> MADRANNDDDVDRQPLPIADDADDDVDGIDEMFNNEDEDPEDEEGENLFGDDMERDYREQPELDQYSESGMDDASDVGSLSVSARRAAEREMAQRDQLLDDDALMYEDGDSEEVDTRRRGRGRRGRGDAADDDSVPMEEEDIPVDILENIRGRTIRDHVSDEAVAKEIERRFKNFLRSFHEPGNKQTKYIQMIKSMAADNRESLEVSFTDLSDDNGEQNISYFLPEAPNEMLAIMDRAATEVVMNMYPFYSRVCNEIKVRISQLPVEEDIRMLRQVHLNMLIRTAGVVTIASGILPQLAVVKYDCVACGYLLGPFVQQNDEEVRPTICPSCQGKGPFELNVENTVYHNYQRITMQESPNKVAAGRLPRSKDVILLGDLCDSCKPGDEIEVTGVYTNNFDGSLNYKQGFPVFNTLIHANHITNKDKMASDQLTDEDIKAIRELSQDPNISQRVFSSIAPSIYGHDDVKRAIALALFRGEAKNPGAKHRLRGDINVLLCGDPGTAKSQFLRYAAHIAPRSVLTTGQGASAVGLTAYVQRHPVTREWTLEAGAMVLADKGVCLIDEFDKMSDQDRTSIHEAMEQQSISISKAGIVTSLHARCTVIAASNPIGGRYNPTRTFAENVDLTEPILSRFDVLCVIRDSVDSVEDERLAKFVVGNHRTHHPDAKKIVKEGDELEEDQMDERTGVRLIPQDLLRKYIIYAREKCHPTLPEQHSEKFSNIFAQMRKESMATGSVAITVRHVESMIRLSEAHAKLHLRSYVNDEDCAAAIRVMLESFVNTQKASIMRMMKKTFSRHLTENRSANELLLFILKQLIRQQMHYATARAAAGTILQSVTIPESEFIEKAQQLRIENVKPFYTSEIFASNNFLYDPSKKTIVQEIF;> MDGQADGMFIDRAEDARKQEITEQYLNFLDNQADTFHYRQKIVKMMNDGESRLVMNLDEIREILPERAEGLLTQSVLEMNCLQSALQMAINRSDVQAVVKTGFHVGFEGTFGERHVNPRTLKSSYLGNLVCCEGIVTKCSTVRQKLLTSVHYCPATNKVLEKKFADFTMLDTAVTNNNYPTEDENKNPLETEFGHSVYKDHQTFTIQELPESAPAGQLPRAVDCVADLDLADRVKPGDRVRIIGVFRVLPNKQNGVSSGSFRSIIIINHIQMLSKEVIPNFEPQDVKDVRKISKSRNPFELLARSLAPSICGHEETKKALLCLLLGGMEKILNNGSRLRGDINVLLIGDPSVAKSQLLRYVLRMAPRAITTTGRGSSGVGLTAAVTTDPDSGERRLEAGAMVLADRGVVCIDEFDKMSDIDRTAIHEVMEQGRVTISKAGIHAKLNARCSVLAAANPVYGRYNPFKSPMENIGMQDSLLSRFDLIFVLLDEHDADKDANVAEHVLKLHTYRTQGEADGTVLPMGGGVETISTINMETKKASSSIYEENTQWAGIQDTKILTMDFMRKYIHLARSVQPKLTDEATEYISEVYADIRSFDITKTDQERTMPVTARQLETLIRLSTAIAKARFSKKVEREDTEKAYNLLHFACFKEKPKARQEYEKKKRAPRIDGDDDEDQSDNEDMATSEEPQSSSVPTAATPRRGVRRRAEDDDSQDSMMDTTIGESQPTAKKARTGPAAIGVDRYKELRKYVRKAFDDIGSTDDMVELQIITDSVQTQAGSHKFTEDELKAGYEQLENDNAAMIAEDKITLI;> MPRSNDPAEPQSESADLFAEPSSQHSSMRSGSEQVAGNMSPRSTSSASALQYGSEMGSVSQMSSASTLRRGGPRGDLGIAAVDHRTVQIRGMEDEMAGDDGQPRLYVWGTRICVADVQRSFRDFLTTFKISQLAEDENMMTGHDEALHEIDVNHPYYMERLLECNDAEVTHINLNLKHLNAFSEALYRKVIAYPADVIPYLDIVVNEVFAERFNRTLAQSIELRPFNAQKTRNMRGLNPNDVDQLITISGMVTRTSSLIPEMRSGYFQCAVCAFGIESEVDKGRIEEPVVCTNCSNTHCFQLVHNRSVFLDKQVVKLQESPDDMPSGETPHTVSVYAHGSLVESVQPGDRITVTGIFRATGMKVNPKQRALASVYRTSIDALHFRKMDTSRLHQDNGETITEERIQQIIELSKRPDIMDALAQSIAPSIYEHDDVKRGLLCLLFGGTRKDDETTNKTKLRSEINILLCGDPGTSKSQMLQYVYRLLPRSQYTSGKGSSAVGLTASVSRDADTKQLVLQTGALVLADNGVCCIDEFDKMNESARSVLHEVMEQQTLSIAKAGIICQLNARASVLAAANPVDSKWNRNKTIVENITLPHTLLSRFDLIFLIVDAQDEMQDRRLGNHLVSLYFENDGNQEKTEHVDMNLLRDYIAYAKANIHPKLSEEASQFIIEKYLFMRKAGAQHGQITAYPRQLESLIRLSEAHAKIRLSQEVSVDDVEKAFTLWREALKQSAVDPSTGRVDVAILASGMSASGRKAVEAMCEAVLKQLKTAKGFVTSKALFHTLKSADKTCQREVFDEAINELSKKESIARSGDRIRFQTEA;> MSNLDNPGIYYQERFFANDGVPDTGRELIAEYRQLITQFRNFIRDFSTGGFGMIYRDQLKRNYFSHEYRLEINLNHLKNFDEDIEMKLRKFPGKVLPALEEAAKIVADEITTPRPKGEEKLHDIQVTLTLDEYPTSLRQVKSAQVSQVVKISGIIVAAAQVRSKATKVTLQCRQCKHTIPDVSIKPGLEGFALPRTCAAPQQGQMQRCPIDPYIMLPDKCECVDYQTLKLQENPEDVPHGEMPRHLQLFTERYLTDKVVPGNRVTIVGVYSIKKLIQKKGGDKSLQGIRTPYLRVLGIHMETSGPGRTNFTTFTPEEERMFKTLAQRKDAYELIAKSIAPSIYGSADIKKSIACLLFGGARKKLPDGITRRGDINVLLLGDPGTAKSQLLKFVEQVSPIGVYTSGKGSSAAGLTASVIRDPQSRSFIMEGGAMVLADGGVVCIDEFDKMREDDRVAIHEAMEQQTISIAKAGITTTLNSRCSVLAAANSVYGRWDESRGDDNIDFMPTILSRFDMIYIVKDTHDVLKDATLAKHVIEVHVNASAAKERDIAGVPKTATTDSDGVMTMFDTDGFLTIEFLKKFVTYARLNCGPRLTPQASEKLVNHYVKMRNPVVNADAFKSGKKAHNSAIPITVRQLEAIVRIAESIAKMELQQFATDKHVEEALRLFRVSTIEAAATGNLAGVEGFTSTADQEALNRIEVQMKKRFAIGTHVSEHLIVQDFVARQHYRESLVKKVIDNLVRRGDLQQKMQRKMLYRVR;> MDNIIGGQAQQVEDTDGTRVQNEFSKFLKSFKDQKNEFIYKSAMKELVQPEKNTIFINMQHLYKFSNNLATTIELQYYRVYPFMCEALHLATLDACDESERQQMFKKQLYVSLFNLDAKTKVRELSADKVGGLVRIAGQIVRTHPVHPELSRACFVCEDCGVTTRDVQQQFRYTQPTKCANPQCMNRTRFSLDVNSSTFVDFQKIRIQETQAELPRGSIPRTVDVIVRGEMVETVQPGDKCDIVGTLIVIPDIAQLSTPGLRAETSNQNRGRATDKSEGITGLKALGVRDLTYKMAFLACHIQQTESLVGGDASGAVEETDYLDLWSKMSTEDRATLKKMSDDKKIEKNIVDSLFPNIYGNHEVKLGVLLMLLGGVAKKSRDEGTSLRGDINVCLVGDPSTAKSQVLKAVEEFSPRAIYTSGKASSAAGLTAAVVKDEESFEFVIEAGALMLADNGVCCIDEFDKMDLKDQVAIHEAMEQQTISITKAGVKATLNARASILAAANPVNGRYDRSRPLKYNVQMSAPIMSRFDLFFVLVDECNEVTDYAIARRILDNHRAISEHTERDSVYKIDDIKKYIAFARCFKPKISDKAAETLVREYKKLRMSDSNNAATSSWRITVRQLESLVRLSEALARLHCGKEVLVEHVEKAAELLNKSIVRVEQPDIALDDDDFDNNIMVVEADKENQRGDDSMDHDGEKENAPKIDIAKLKISFKEYKQLSDVLVLHMRSDEDNQGEDEYDGVKQSALVEWYLSTIEADLETEEDFNVQKTICERVIHRLIHQDHVLLEVEQGEDPTLCVHPNYVIADE;> MKTTTYNTDWAAEKTKIRSFFDEYYVDNEDGSGKAFPYRDQVFEIARRDKQAIVVNVDHIKESDIPDALELSEAITSNTKRYEVLFKDTISDMIQDYLGDKQAPVIDALDAYMFQRLHMDRNEGAANEEVSLQDKRKKYPPQLLQRFEVYFTTDDAAHETCVRNIKATEIGHLVSMKGVVIRATEVKPCVEVMTYTCDTCAAEVYQPVKGMQFTPPVNCPNKECVEAKANGRLHMQLRGSKFVKFQELKIQELSEQVPVGSIPRTMTVHVYGEMTRKCNTGNVVHVSGVFLPIMQSGFRPTGGLVADTYLEAHYINNLDDNPTFNGVQSAELEVLRRKGDNYETLAASIAPEIFGHVDVKKCLLMALVGGNDNSSNGMKIRGCINVLMMGDPGVAKSQLLGYVNRLAPRSQYTTGRGSSGVGLTAAVMKDPVTGEMSLEGGALVLADGGICCIDEFDKMMDHDRTAIHEVMEQQTISIAKAGIMTTLNARTAIIAAANPAYGRYNPNRSIEQNVDLPAALLSRFDLILLMQDKADRENDKILAEHITYVHQHGCHPNREKKDLISLETLREYISLCKTYTPTVDPALRERIVEAYVEMRRDARYSSDPTFVSPRMILGIVRMATARAKLRLSTIVDESDVEEALRLMQFAKDSLRPEQNKIEKRMAPVDAAFAVLRELYHADNAPIAISNAIQRCARKGISEVALKKCLDQYTANGLLVMDRQNIVFAMN;> GPGSMSSGDQNRGGVADKALQLVLEMKRNPDVLPPYNTELVRQCYQKIDELFQKNAAVVEKIRAGLPHDSTLLQPRLAAMCHIRRCMMAYVNERKNRIRSFRWKYGGALPASVRNALCDAEIQFFNEYSSTLARFQSNLGEGGVNLLLHSAPPKSLFVQVRALEDYGEFETSDGTQVQLSKDSLHSLPRQDCEMLIRQGVLELVH;> MNAERCEFIAGNSLIEVIPSISDDRPIHLISGDIGPFEAGVPCRIPVWTAILMKRKHNCKVVAPQWMDVDELKKILTSETESQGLAKLPDHFFEISHMLVRDAREDIFEVEAVKSLVQDIYDRRDAKLRSSAIEFLRQNQTCHAQLDNVQLIEASSARATLEACRQMGAVVRNKHESTPL;> MAGFEIQRVESKFFDLDDIIAKSDSTSCTFEIGDLNPDFFQEMLGVSKPTQNADGYGVDAPYWLLESVRSSFSIQLPKAYSVNMQNVLNADSKKLNLSGLQQHFYGNGMQLCRLMKGENPDGALSLARCLVSTLTQRLGEIVSTATHLQSKGEKFDSLETKVFLEGKRCKEDIDTWLRQDNKCSSKKRKRLSL;> MAVTDSATTFLDFDDDEYDEMTTPEEVLRKMTATWQNELCAPCLLPTQMELVEILLDQIQGMEENIGKQTDKMQLRISVHRVELQRIGFITSDYVRCRLQKIESNPHDAIDQHKKRKEEGKSDLLSESEMKFAEEYALAESNLFQKTVLEFMPAALKKMPVPRGDHDDVMVYAKVTSDDVGNVAIPDWQDLNGEVILEMEPESCHLIPFESVHQLVEDGNIQLM;> MIIEDNFRQEFYNKIKKGDKSVVLIVSVDTDALCTTMILTHLLRCDDIPFSILAVEGWSSVEKIFADSQEQKCHYILINCGATRSLTRLQIPPASIAFVIDSHRPFHIENVYENGQIHLLANPSEMSELQIPDLESVIREDSDDEEDSDEDEDQEYISYEQRMEKIRRKAIKREEMQIWERQRRTILWRYYESTWFSSPSCVTLLEMAAEMNRVSAETMWFTAVGLNSAMADKLISIEMYTQICVDRMRPFVHRFMPKNIVNQGKVDDLLHITFGRELPLALYSHWDLFSAMMVSEYFSIKTKNWTQKGDVNIRHLLAQLGITLHETKQKFEALPTEQRNLVVDVLEKEMDSSFATFFGTLGYCGKLSACDVARAVTLRLEMPKSETIMNRFRSGQSILRSSITGERQDRLNLNNTFTSICQRTLQVSWKTVAAAINQSEIIPNGPYYLFSCSRSIDEDMVDSRHFLYNTAGFMIRAFASMKKGRTTKPLIAMFPLTGESAGWLVVTGVMPIATIYEDSLLKTCIGRAFERVKKMTPPLRIVDDYFNSDIIRLKSEDRTRFIDFLQTVFEGTSN;>MSDEHYNPRNRLKTQIKRRSSCRNILNAVPPPPPTDFEGLEGFTDSCPAPTANNPFKVSSPQKKRQKPQVTFSQDDPFAASISRSPDPLKTPTKGVRSSPRKRKSPQKFERFQSFDPALLQEFHPVDFSALLATSSSAQKPAEPAQESAEDLPTDLRIGSKMRIVSKVSFPWMNTRKSTGNVIVKFQTNDRFDGMQYFNKTFLNGYEDPTVPLPVSPMSILEAASLFYQFPVIPGLKMYPRITAEQENVSRVSLAPLVTSTMLEQWQECYAELYSSYKKGQRGSFYVATAVCNVLFTKMPLSGGGDDVAADDTSQSCSQAFRGQKLVAVITHTTSAIREHLRSQGVDFEAPKPTSSLKRVSSSPQLHHDQSTLDCLLASESKENSQMGPTTFGGIENSENSDESPLKKDQDSDENESPMKLANQWLNEIGVSPRTVKNTVSRELSSQVTDRAGFQCLVVHGSKIHALFNALMDSDVVHEKTGPYTKIPPTLIATSPFLYGQLLSLTKSSNIFAKAGTKCTEYELKLENGPVLPHCAKMMTQFIRSTNMCSTEEKPVTMQVMDRHTSQGMSDWTETATNWNTVTIAENCVKWTKN[3x];> MNVLVQGAVHALGYYEDGKYSREPDCYESIRDLIRYLREDGDDHTARIECGRHNLVEQDLVPMVKCEDLTDDEFDIAIRLMVNLCQPAISTMRGKPPADRDQWKMYWELEENLRRAKTAFSDAHFFTAIKKRIDNYFIDTEYEDRDERLRLVVERIVLLIKYVFSINPDTSEGRRTRIEDSSHDRVIIAFLESGIDKTLMHIANQPREKEFHVTILDIFALILKEQTAEDLATKSEEVSTAEQKKTEEEFRKIIENHVVKETQKRKSFSRFGGSYTIKGLKGISANSSQVVFKPIQNVEKHNFLDDRKAKKRAPRNRRPFEIDTNSHFASSEVRGMLRDMVIRIIETCFNRLMKSSKTTVFVQVQKTSQINYFFLIKFVLRFVRLSRQDHLLERISECIGVEAFHENNVQLTEYVENATTLKGVEAKSHGLKAQYALGAYNELVLLHRYIYEHAKEENERKFAKRALEHIVNVEEYRELPIFIIKKFSSSVLSNNFLRELVLTTHHYMKLVERFVKTGALKKVTKKVKVRKATKKSKMSEEDVRSEFDGMSKKDLDRLWEESKGLVLQILKKEVPEMRGMNPIDSQLDVPVDAQQKFAKLSIQRSLRSRGFPAAVGLYHASRALWPESFKRGLTDFQDSPGEEDQLQELEQLLKADMKKVAKDLKKAESCKTCDEDPAYKKYDKMDATALQSLWEQSTDTLARILSHELPESESTSPVNWQLDITPDVQQKFAMLAIQRALRARDLPAAVGLYHTSRKLWPGDEAIFGAPGIGVEEEIAELKAILEADLHEVAREMKVAEDRAEDPDEEDPAEPYDSEQEEEEEVPAWKVEEIDFQFDSYVCKFSNVDVLKWYVFLLNDFSKNSTELNQALVKMLHRIAFDLKLPIKLYQVSLFQVFSKVNEHFTHLSKDLRKSSRLYELYQFGFHLLKKFFSKFTGDLAIEALFWKGPRECFEIENGYGSWVKSREADIRVWTEDLEIELRNLYEEYRTMETRDGIDVLDFIEHNLSRARSRKKVAKKLIEFGFDLLGAKWKNSDKARMDSVLPIGDIQKWYDEWKEAGARGDLVNVLQEKLNEDLGMEISRKKILKQLAHMDILYEKPKKEKPLPQWDTGLIEELKKLKEQYDDIPDALNMLGVNIVRYVMKRLSEKKPTRQVERHLESLGATIPERSKKSEKNGKKFDDFLNDDDDDSENDVGGGSEDDEEEEIVMKSKRIIPDSEDEEEHIEQEEAQKKLEKVAEKPNTLMGMIAGRKRKLAQLESDSSDESDDDDSAEKEEKKLPAAEDDSDLEEDAVIYKRSYVDALLTGGSIAGNGITETRRDTSEEREDDDDEDPFTKKLTFKRRIVMSDNEDEA;> GPGSMDEMEDFFENDELDREPSPMGDEAIEDNSGEGGTRRVVEPKLLRTKRLANPRLALNERILTGPKGISALRETLKDFKPNPKDDPYANLEKLMKKYAYWGHLMFPKMKTEDVLNRVETLGTRRQVKVFMIKHRLGETGEDSEHEEQENQKNGIIDDGASDNDDDLFKDLPEKEVTTEKAKNSEKSDQKTAEIDENVEEEYRMMEEERLREEQEAKEAADEDALMEDFGDMNNDW

The key regulated step during initiation is the assembly at multiple replication origins of the DNA helicase known as CMG (CDC45-MCM2-7-GINS), around which the replisome assembles. CMG unwinds the parental DNA duplex at a replication fork and associates stably with the DNA template until neighboring forks converge during DNA replication termination. Here we show that the Caenorhabditis elegans protein DNSN-1 is essential for replication initiation and acts together with MUS-101 during CMG helicase assembly. Our data indicate that DNSN-1 binds simultaneously to GINS and to the MCM-3 subunit of MCM-2-7 double hexamers, thereby positioning GINS in a precise fashion to promote CMG assembly.

The association of DNSN-1 with the CMG helicase was then analyzed by cryo-electron microscopy (EM), in the presence of replication fork DNA as well as a complex of TIM-1 and TIPN-1 that was included to stabilize association of CMG with DNA. The resulting structure, which was determined using cryo-EM density maps with average nominal resolutions of 2.6 Å – 3.8 Å (FSC = 0.143 criterion), confirmed the existence of a DNSN-1 homodimer that associates with the GINS and MCM-3 components of the helicase. Specifically, the folded domain of one protomer of the DNSN-1 dimer forms a large interface on the amino terminal (forward-facing) side of the MCM-2-7 motor of the CMG helicase. In this way, extensive interactions with the PSF-2, PSF-3 and SLD-5 subunits of GINS serve to position the DNSN-1 dimer on CMG, together with further interactions with the MCM-3 amino terminal domain (Figure 7C (i), NTD, N terminal domain). In addition to the folded domains of the DNSN-1 dimer, cryo-EM density corresponding to an α-helix is observed at two other positions within the complex. Firstly, one α-helix is bound to a distant region of GINS beside the N-terminus of SLD-5, where it contacts SLD-5 and PSF-2. Aided by an AlphaFold-Multimer prediction, the amino terminus of DNSN-1 (residues 4-19) can be unambiguously modelled into this density (Figure 7C (ii), Figure S13A-D). The interaction of DNSN-1 with the MCM-3 AAA+ domain and the MCM-3 NTD, in addition to multiple GINS subunits, likely explains the greater affinity of DNSN-1 for CMG compared to isolated GINS.>[2x]MKKIPCVMMRGGTSRGAFLLAEHLPEDQTQRDKILMAIMGSGNDLEIDGIGGGNPLTSKVAIISRSSDPRADVDYLFAQVIVHEQRVDTTPNCGNMLSGVGAFAIENGLIAAT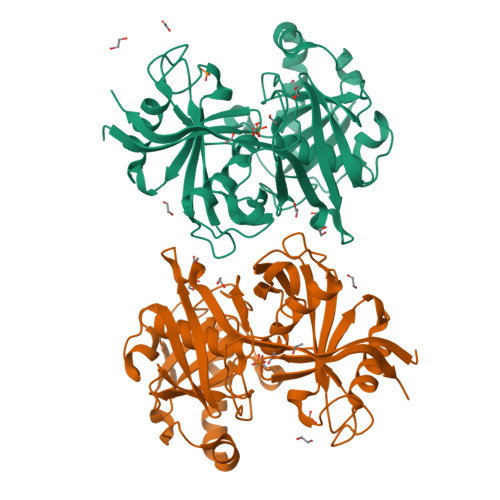SPVTRVRIRNVNTGTFIEADVQTPNGVVEYEGSARIDGVPGTAAPVALTFLNAAGTKTGKVFPTDNQIDYFDDVPVTCIDMAMPVVIIPAEYLGKTGYELPAELDADKALLARIESIRLQAGKAMGLGDVSNMVIPKPVLISPAQKGGAINVRYFMPHSCHRALAITGAIAISSSCALEGTVTRQIVPSVGYGNINIEHPSGALDVHLSNEGQDATTLRASVIRTTRKIFSGEVYLP Transketolase (TK) (EC 2.2.1.1) is a ubiquitous thiamine diphosphate (ThDP)-dependent enzyme linking the non-oxidative pentose phosphate pathway and the Calvin cycle. It catalyses the reversible transfer of a two-carbon moiety from a ketol donor to an aldehyde acceptor. Transketolase has been used to form asymmetric carbon-carbon bonds in biocatalytic organic synthesis, where the use of β-hydroxypyruvate (HPA) as the ketol donor renders the donor half-reaction irreversible. A different library design strategy was used at each stage to guide saturation mutagenesis, including the use of structural and phylogenetic information, statistical coupling analysis (SCA) methods to target networks for re-stabilisation, and substrate docking. In the latter stage, saturation mutagenesis of two TK active-site residues led to variants, including S385Y/D469T/R520Q, that were active on three benzaldehyde derivatives, in contrast to wild-type TK which was active only on non-aromatic aldehydes.

The crystal structure of S385Y/D469T/R520Q E. coli TK in the presence of its cofactors was determined to 1.50 Å resolution with very good statistics (Rwork: 12,58%, Rfree: 15,69%). The structural analysis of EcTK S385Y/D469T/R520Q could unambiguously confirm the introduced mutations. In fact, there was no evidence of any significant shifts in backbone, sidechain or cofactor structure compared to the wild-type protein. The aromatic side chain of introduced residue Y385 is accommodated almost coplanar 7–8 Å above the thiazolium ring of ThDP thus generating a snug π-π stacking binding pocket for aromatic substrates (sandwiched between Y385 and ThDP). The binding of aliphatic phospho-sugar substrates is clearly impeded as the Y385 side chain would clash with the substrate phosphate moiety, and the S385Y mutation also removes a hydrogen-bonding site to the S385 hydroxyl moiety, which is known to interact with phosphate groups in the natural substrates of TK28. In the triple variant, the side chain of Y385 is held in place through a network of H-bonding interactions involving 3 water molecules and residue G262. The D469T mutation removed a salt bridge to R91, and replaced it with a hydrogen bond from the T469 hydroxyl moiety. The mutation also created a small pocket in which the R91 guanidinium moiety is more solvent accessible within the enzyme active site, and also available for hydrogen bonding to potential substrates. The R520Q mutation created a wider opening to the active-site funnel, which may compensate for the decreased steric access for substrates, introduced by the S385Y mutation. Introduction of the S385Y mutation into D469T/R520Q to produce the triple-mutant creates an enclosed hydrophobic binding-pocket for all three benzaldehyde substrates.

>[2x]MSSRKELANAIRALSMDAVQKAKSGHPGAPMGMADIAEVLWRDFLKHNPQNPSWADRDRFVLSNGHGSMLIYSLLHLTGYDLPMEELKNFRQLHSKTPGHPEVGYTAGVETTTGPLGQGIANAVGMAIAEKTLAAQFNRPGHDIVDHYTYAFMGDGCMMEGISHEVCSLAGTLKLGKLIAFYDDNGISIDGHVEGWFTDDTAMRFEAYGWHVIRDIDGHDAASIKRAVEEARAVTDKPSLLMCKTIIGFGSPNKAGTHDSHGAPLGDAEIALTREQLGWKYAPFEIPSEIYAQWDAKEAGQAKESAWNEKFAAYAKAYPQEAAEFTRRMKGEMPSDFDAKAKEFIAKLQANPAKIASRKASQNAIEAFGPLLPEFLGGSADLAPYNLTLWSGSKAINEDAAGNYIHYGVREFGMTAIANGISLHGGFLPYTSTFLMFVEYARNAVRMAALMKQRQVMVYTHDSIGLGETGPTHQPVEQVASLRVTPNMSTWRPCDQVESAVAWKYGVERQDGPTALILSQQNLAQQERTEEQLANIARGGYVLKDCAGQPELIFIATGSEVELAVAAYEKLTAEGVKARVVSMPSTDAFDKQDAAYRESVLPKAVTARVAVEAGIADYWYKYVGLNGAIVGMTTFGESAPAELLFEEFGFTVDNVVAKAKELLHHHHHH> ELTPDQQTLLHFIMDSYNKQRMPQEITNKILKEAFSAEENFLILTEMATNHVQVLVEFTKKLPGFQTLDHEDQIALLKGSAVEAMFLRSAEIFNKKLPSGHSDLLEARIRNSGISDEYITPMFSFYKSIGELKMTQEEYALLTAIVILSPDRQYIKDREAVEKLQEPLLDVLQKLCK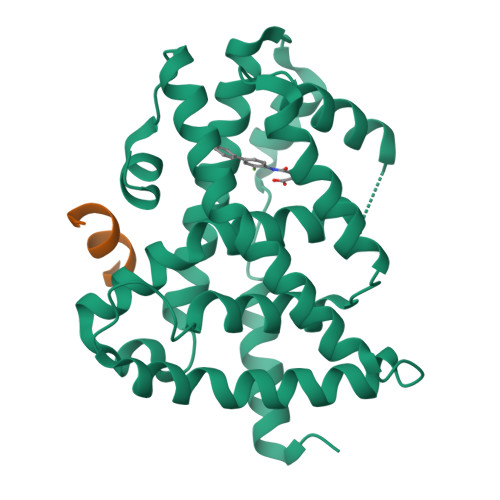IHQPENPQHFAKLLGRLTELRTFNHHHAEMLMSWRVNDHKFTPLLQEIWDV;> NALLRYLLDK> MSGRLGELLVRENLISVQQLRKAQEEQQKNGTRIGTALVKTGAIEESKLTDFLSKQYGVPAINLKDFDVEPDIIKLVPKEVAEKHLVVPVNRAGPSLIVAMCDPSNIFAVDDLKFLTGYNIETVVASEVSIREAIERYYAEKGPSLEDIVGDVGDDIEVTKEETENIDEMAKAADDAPVVKLVNLILMDAIKKRASDIHVEPYEKDFRVRFRIDGVMYEVMRPPMKLRNAITSRLKIMASLDISERRLPQDGRIKIKMGGGKEMDFRVSVCPTLFGEKVVMRLLDKSNLQLDMTKLGFDAQPLAWFKEAIDRPYGMVLVTGPTGSGKTTTLYSALSSLNGLDTNICTAEDPVEFNFAGIN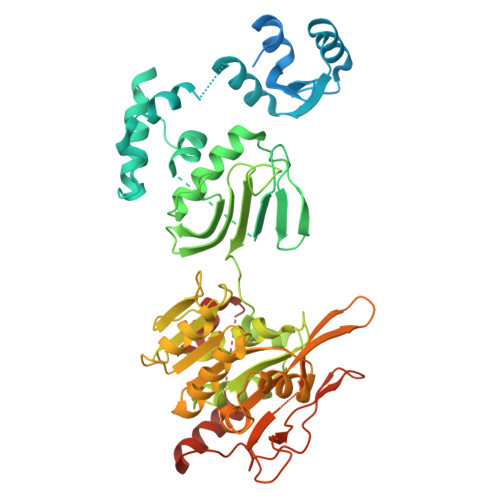QVQMHDDIGLNFAAALRSFLRQDPDIIMIGEIRDFETAEIGVKAALTGHLVLSTLHTNDAPGTVSRLLNMGIEPFLVTASLNLILAQRLARRLCPACKKPAENVDEQALIDAGVPPDKIGTFTMYEKVGCRDCNDRGYRGRVAIYEVMPFWDGLKELVINGASAAELKQEAIRLGMSSLRMSGLRKMMDGATTLEEVVGNTAPDRF> GSHMLELPHEKDKPVAEPIPICSFCLGTKEQNREKKPEELISCADCGNSGHPSCLKFSPELTVRVKALRWQCIECKTCSSCRDQGKNADNMLFCDSCDRGFHMECCDPPLTRMPKGMWICQICRPRKKGRKLLQKK

The developmental regulator monocytic leukaemia zinc finger protein (MOZ) also known as (MYST3/KAT6A) is a MYST (Moz, Ybf, Sas, TIP60) family acetyltransferase that is required for self-renewal and differentiation of haematopoietic stem cells. In addition to the MOZ acetyltransferase domain (referred to as the MYST domain), the N-terminus of MOZ contains two tandem PHD fingers comprising the double PHD finger (DPF) domain. The structure of MOZ DPF shows the typical globular domain of a DPF with PHD1 and PHD2 each harbouring two zinc atoms coordinated by C4-H-C3 motifs in cross-brace topology. The structures combined with biochemical studies reveal how MOZ DPF manipulates the structure of the H3 tail to sample its modification status and promote its acetylation.

To understand the molecular basis of H3 recognition by MOZ and the consequences of H3K9 and H3K14 acetylation, we determined crystal structures spanning MOZ DPF (194–323) alone and in complex with a series of histone H3 peptides (1–21), unmodified or acetylated at H3K9 or H3K14 to 3.0 Å, 1.6 Å, 1.6 Å and 2.5 Å resolutions, respectively. In our structures, residues L194–D199 at the N-terminal boundary of PHD1 form a helix (denoted as α1) that folds back onto the DPF core and interacts with the PHD2 subdomain through salt bridge interactions between E197 and R286, hydrophobic contacts engaging L194 and I309 and interactions between the H196 and R269 side chains. Other interactions between the PHD1 and PHD2 subdomains are observed, including a hydrogen bond between W257 and D285. On H3 binding, subtle conformational changes in the DPF domain occur in regions of direct contact with H3, including a side chain rotation of F280 and changes in a linker region (designated L1), which harbours a helical turn in the H3 complex (A275-N277; labelled as α3a in Figure 2B) but not in the unbound DPF structure. The side chain of H3K4 inserts into a pocket on the surface of MOZ DPF that is partially occluded by residues from the L1 linker in the unbound DPF crystal structure.> MQGEIIAGFLAPHPPHLVYGENPPQNEPRSQGGWEVLRWAYERARERLDAMKPD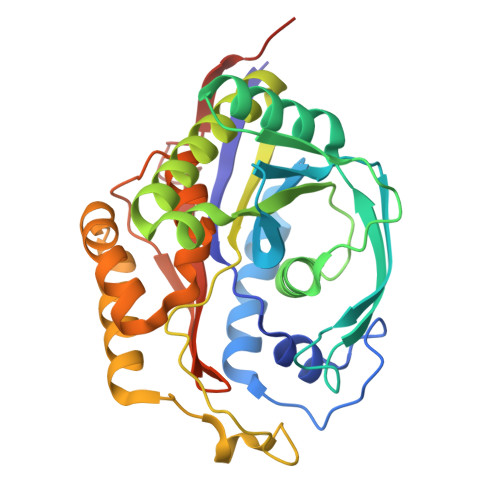VLLVHSPHWITSVGHHFLGVPELSGKSVDPIFPNVFRYDFSLNVDVELAEACAEEGRKAGLVTKMMRNPKFRVDYGTITTLHLIRPQWDIPVVGISANNSPYYLNTKEGMSEMDVLGKATREAIRKTGRKAVLLASNTLSHWHFHEEPTIPEDMSKEYPATMAGYQWDIRMIELMRQGKTSEVFKLLPQFIDEAFAEVKSGAFTWMHAAMQYPELAAELFGYGTVIGTGNAVMEWDLRKAGLSMLGAADQKQRSAAVA>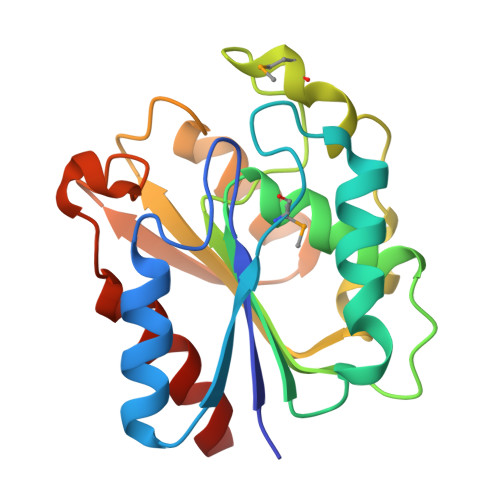 GRGTKQVYIIHGYRASSTNHWFPWLKKRLLADGVQADILNMPNPLQPRLEDWLDTLSLYQHTLHENTYLVAHSLGCPAILRFLEHLQLRAALGGIILVSGFAKSLPTLQMLDEFTQGSFDHQKIIESAKHRAVIASKDDQIVPFSFSKDLAQQIDAALYEVQHGGHFLEDEGFTSLPIVYDVLTSYFSKETR>GSHMAEVHHWSYEGENGPENWAKLNPEYFWCNLKNQSPVDISDNYKVHAKLEKLHINYNKAVNPEIVNNGHTIQVNVLEDFKLNIKGKEYHLKQFHFHAPSEHTVNGKYYPLEMHLVHKDKDGNIAVIGVFFKEGKANPELDKVFK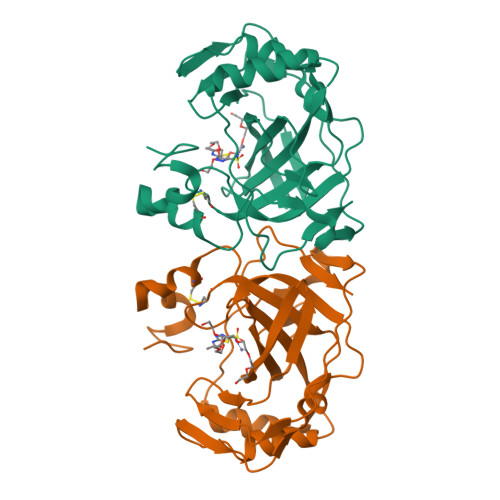NALKEEGSKVFDGSININALLPPVKNYYTYSGSLTTPPCTEGVLWIVLKQPITASKQQIELFKSIMKHNNNRPTQPINSRYILESN[2x]>PFTEIKSGFLERRSKFLKSYSKGYYVLTPNFLHEFKTADRKKDLVPVMSLALSECTVTEHSRKNSTSSPNSTGSDAKFVLHAKQNGIIRRGHNWVFKADSYES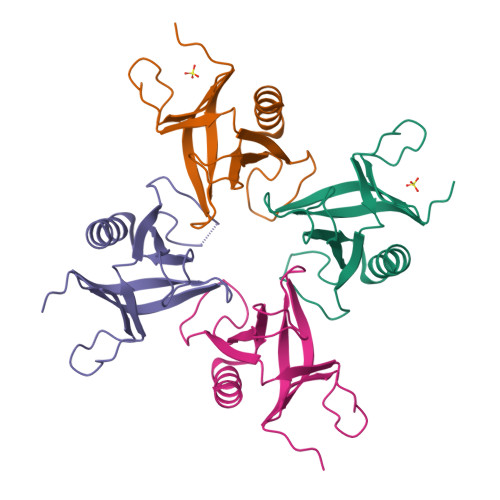MMSWFDNLKILTSTS[4x]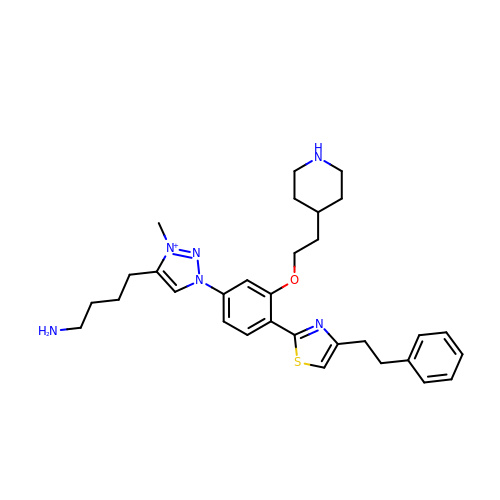4-[3-methyl-1-[4-[4-(2-phenylethyl)-1,3-thiazol-2-yl]-3-(2-piperidin-4-ylethoxy)phenyl]-1,2,3-triazol-3-ium-4-yl]butan-1-amine | C31 H41 N6 O S | HGXOIGOGRBONFR-UHFFFAOYSA-N> ANIQSFSFKNFNSPSFILQGDATVSSGKLQLTKVKENGIPTPSSLGRAFYSSPIQIYDKSTGAVASWATSFTVKISAPSKASFADGIAFALVPVGSEPRRNGGYLGV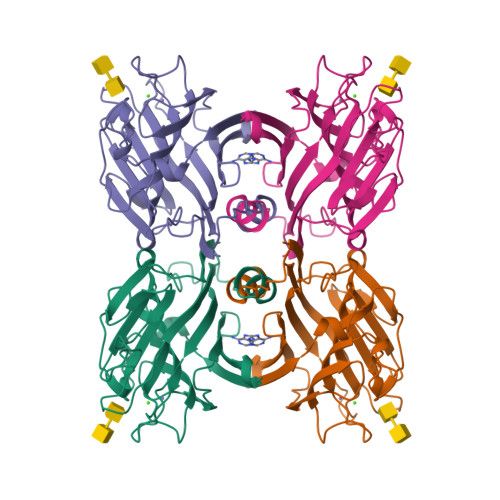FDSDVYNNSAQTVAVEFDTLSNSGWDPSMKHIGIDVNSIKSIATVSWDLANGENAEILITYNAATSLLVASLVHPSRRTSYILSERVDITNELPEYVSVGFSATTGLSEGYIETHDVLSWSFASKLPDDSTAEPLDLASYLVRNVL> GSLDGPYAPDSSNLPSNCWYLVNPSNDGVVFSVTDNSTFWMFTYLVLPNTAQTNVTVNVMNETVNISIDNSGSTYRFVDYIKTSSTQAYGSRNYLNTAHRLQAYRRDGDGNISNYWGADTQGDLRVGTYSN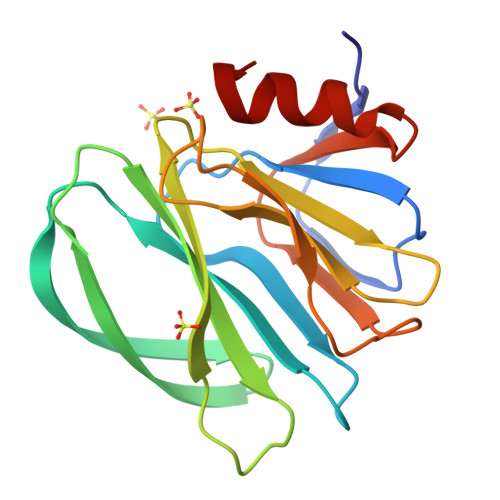PVPNAVINLNADFYVIPDSQQETCTEYIRGGL> NSQPIVAPRTAEMQGDPFGLLLRQRIVFLGGEVEDFGADAIISQLLLLDSQDPTKDIKIFINSPGGSVTAGMGIYDAMMLCRADVNTYCFGLAASMGAFLLGAGKRGKRNSMPNSRIMIHQPLGGASGQA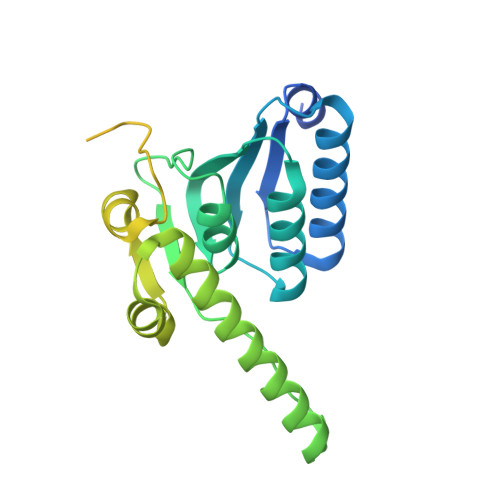VDIEIQAKEIMYHKANLNRIMADYCQQPLSKIEEDTDRDRYMSPLEAKEYGLIDHIIGGEEAVFNVKGSLKKFPKIKEEFVTDKDDMVKRNIMDGDPFLSETPSWRFKSPQTEPYMPSQAPGSRWFRTRKVSKEDYKEMQEQRQAELMAESDDGKKSVKDRIDDAW>MTLDNSKEELKGHKGINLPPKFSADYDTKLSAEEIATLEKTALEMNKNFPTSKEDEKNKDVMWDIQHLSADQKKELSVYTTELLNDVRKKLGLSQLSVSDQSIKFAWDIAKYSDTGEYMHDVIAINKAAKENGFKEYP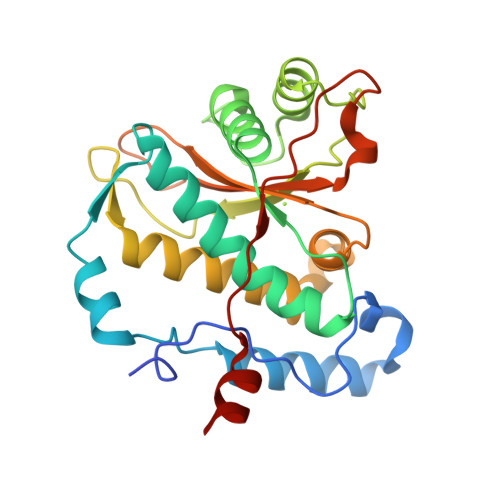GMNYYENLGGGYYETENGKVSKYTLQESIRKMLVNMLFDDGRLGYSHLHSLLQDGKTALGVSLSGEKNSISPKIHIISYGKEKLEDSSQYQNGEVASMKSKEELQQEIASN[2x]> MNSPISPIETVPVKLKPGMDGPKVKQWPLTEEKIKALVEICTEMEKEGKISKIGPENPYNTPVFAIKKKDSTKWRKLVDFRELNKRTQDFWEVQLGIPHPAGLKKKKSVTVLDVGDAYFSVPLDEDFRKYTAFTIPSINNETPGIRYQYNVLPQGWKGSPAIFQSSMTKILEPFRKQNPDIVIYQYMDDLLVGSDLEIGQHRTKIEELRQHLLRWGLTTPDKKHQKEPPFLWMGYELHPDKWTVQPIVLPEKDSWTVNDIQKLVGKLNWASQIYPGIKVRQLCKLLRGTKALTEVIPLTEEAELELAENREILKEPVHGVYYDPSKDLIAEIQKQGQGQWTYQIYQEPFKNLKTGKYARMRGAHTNDVKQLTEAVQKITTESIVIWGKTPKFKLPIQKETWETWWTEYWQATWIPEWEFVNTPPLVKLWYQLEKEPIVGAETFYVDGAANRETKLGKAGYVTNRGRQKVVTLTDTTNQKTELQAIYLALQDSGLEVNIVTDSQYALGIIQAQPDQSESELVNQIIEQLIKKEKVYLAWVPAHKGIGGNEQVDKLVSAGIRKVL;> MAGHHHHHHGSAENLYFQGPISPIETVPVKLKPGMDGPKVKQWPLTEEKIKALVEICTEMEKEGKISKIGPENPYNTPVFAIKKKDSTKWRKLVDFRELNKRTQDFWEVQLGIPHPAGLKKKKSVTVLDVGDAYFSVPLDEDFRKYTAFTIPSINNETPGIRYQYNVLPQGWKGSPAIFQSSMTKILEPFRKQNPDIVIYQYMDDLYVGSDLEIGQHRTKIEELRQHLLRWGLTTPDKKHQ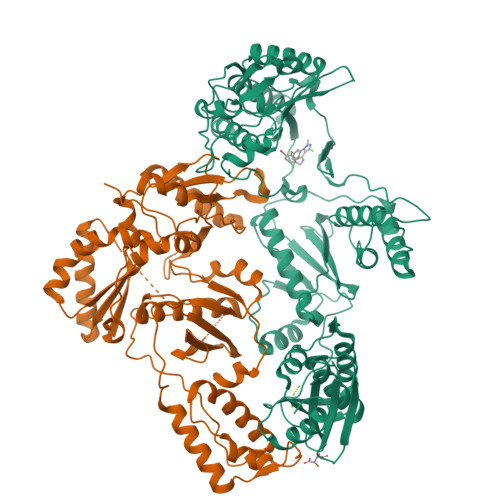KEPPFLWMGYELHPDKWTVQPIVLPEKDSWTVNDIQKLVGKLNWASQIYPGIKVRQLCKLLRGTKALTEVIPLTEEAELELAENREILKEPVHGVYYDPSKDLIAEIQKQGQGQWTYQIYQEPFKNLKTGKYARMRGAHTNDVKQLTEAVQKITTESIVIWGKTPKFKLPIQKETWETWWTEYWQATWIPEWEFVNTPPLVKLWYQ>GGSRCQRDHLSTKLIPTEVPADLIRAVTCQVCDHLLSDPVQSPCRHLFCRLCIIRYTHALGPNCPTCNQHLNPSHLIKPAKFFLATLSSLPLLCPSEECSDWVRLDSFREHCLNHYREKESQEEQTPSEQNLDGYLPVNKGGRPRQHLLSLTRRAQKHRLRDLKNQVKTFAEKEEGGDVKSVCLTLFLLALRAGNEHKQADELEAMMQGRGFGLHPAVCLAIRVNTFLSCSQYHKMYRTVKATSGRQIFQPLHTLRNAEKELLPGFHQFEWQPALKNVSTSWDVGIIDGLSGWTVSVDDVPADTISRRFRYDVALVSALKDLEEDIMEGLRERALDDSMCTSGFTVVVKESCDGMGDVSEKHGSGPAVPEKAVRFSFTIMSISIRLEGEDDGITIFQEQKPNSELSCRPLCLMFVDESDHETLTAILGPVVAERKAMMESRLIISVGGLLRSFRFFFRGTGYDEKMVREMEGLEASGSTYICTLCDSTRAEASQNMVLHSITRSHDENLERYEIWRKNPFSESADELRDRVKGVSAKPFMETQPTLDALHCDIGNATEFYKIFQDEIGEVYQKPNPSREERRRWRSTLDKQLRKKMKLKPVMRMNGNYARRLMTREAVEAVCELVPSE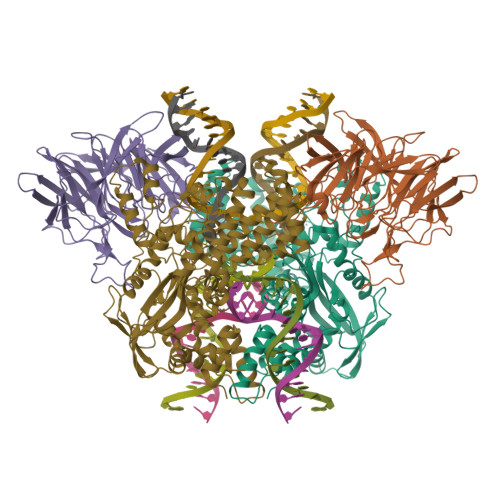ERREALLKLMDLYLQMKPVWRSTCPSRDCPDQLCQYSYNSQQFADLLSSMFKYRYDGKITNYLHKTLAHVPEIVERDGSIGAWASEGNESGNKLFRRFRKMNARQSKTFELEDILKHHWLYTSKYLQKFMEAHKNS[2x];>[2x]GGSMSLQPLTAVNCGSLVQPGFSLLDLEGDVYLFGQKGWPKRSCPTGIFGVRIKKGELKLRAISFSNNSSYLPPLRCPAIAHFEAQDGKPECYLIHGGRTPNNELSSSLYMLSVDSRGCNRKVTLRCEEKELVGDVPSARYGHTLSVINSRGKTACVLFGGRSYMPPTERTTQNWNSVVDCPPQVYLIDLEFGCCTAHTLPELTDGQSFHVALARQDCVYFLGGHILSSDCRPSRLIRLHVELLLGSPVLTCTILHEGLTITSAIASPIGYHEYIIFGGYQSETQKRMECTYVGLDDVGVHMESREPPQWTSEISHSRTWFGGSLGKGTALVAIPSEGNPTPPEAYHFYQVSFQKEQDGEATAQGGSQESTDFEDSAPLEDSEELYFGREPHELEYSSDVEGDTYNEEDEEDESQTGYWIKCCLSCQVDPNIWEPYYSTELTRPAMIFCSRGEGGHWVHAQCMELPESLLLQLSQDNSKYFCLDHGGLPKQEMTPPKQMLPVKRVPMKMTHRKAPVSLKMTPAKKTFLRRLFD> GSLKGTQSLNPHNDYCQHFVDTGHRPQNFIRDVGLADRFEEYPKLRELIRLKDELIAKSNTPPMYLQADIEAFDIRELTPKFDVILLEPPLEEYYRETGITANEKCWTWDDIMKLEIDEIAAPRSFIFLWCGSGEGLDLGRVCLRKWGYRRCEDICWIKTNKNN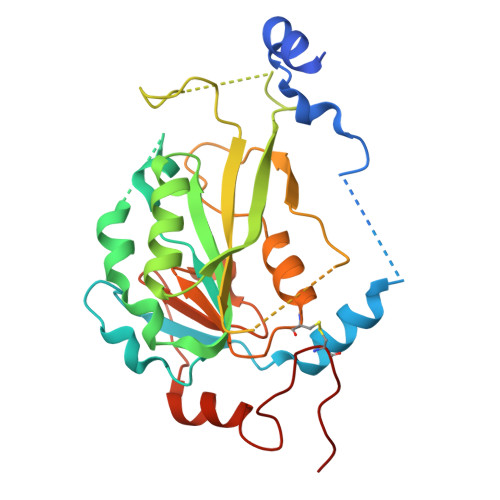PGKTKTLDPKAVFQRTKEHCLMGIKGTVKRSTDGDFIHANVDIDLIITEEPEIGNIEKPVEIFHIIEHFCLGRRRLHLFGRDSTIRPGWLTVGPTLTNSNYNAETYASYFSAPNSYLTGCTEEIERL> MSDERYQQRQQKVKDRVDARVAQAQEERGIIIVFTGNGKGKTTAAFGTAARAVGHGKNVGVVQF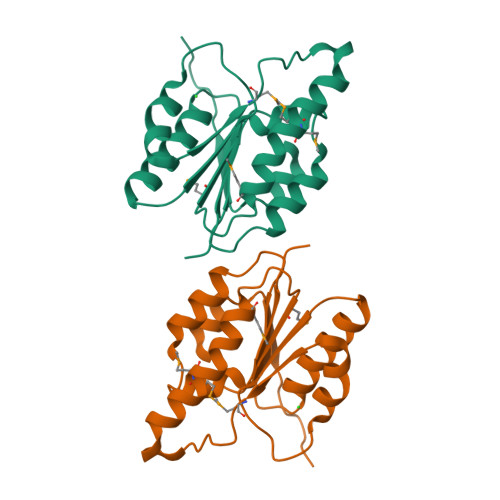IKGTWPNGERNLLEPHGVEFQVMATGFTWETQNREADTAACMAVWQHGKRMLADPLLDMVVLDELTYMVAYDYLPLEEVISALNARPGHQTVIITGRGCHRDILDLADTVSELRPVKHAFDAGVKAQMGIDY>LTTSLEQDPDEQDANREIAAATKQTVETLMAGERIAEALELGMTDLNTIREWEEARQINPNIAPPQRNPIFVALGNIPAETYVLNTLQKIKPASLHDALLVLPFSTIPSLLTFLNLFAQRELNVPLTCRILFFVLKTHHKQIVASRTMRATLEKVRANLRAALRRQKDEMGFNIAALKVVSMQLR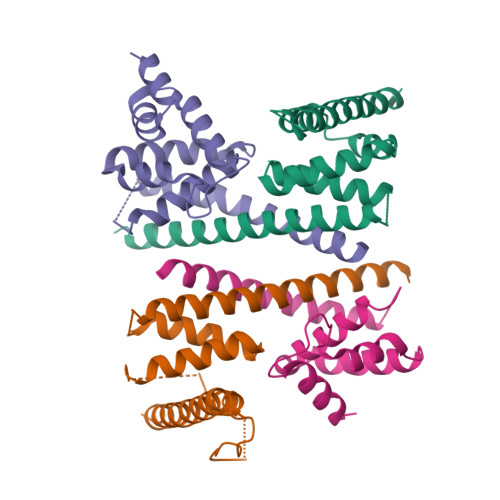DKSVREYVDETWEEKEKEKGVRKR[2x];>[2x]LVEQEQTLENYIHAGAYRDAIVLALQLNHPGRLLNLFTNVVTTRNPDPDSLTGLKAVDDVLAKLSDEQIFQLLLRLRDWNTNARTAPVAQRVLWALFKSHPANKLSSLSVKGARGHKSLNEVLDAIKVYTERHYKRIEELVDESYLVEYTLREMDALTPQTEALEAGEDAVIAEA> ASP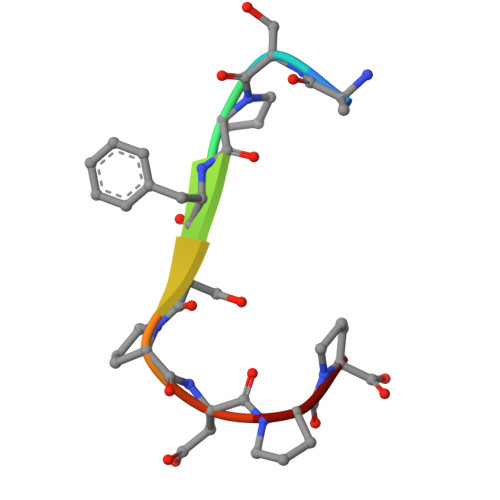FSPDPP>SMLGRLNHVAIAVPDLEKAA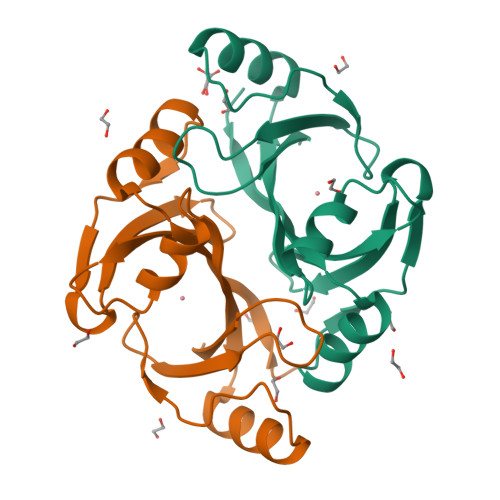AFYKNILGAQVSEAVPLPEHGVSVVFVNLGNTKMELLHPLGLDSPIAGFLQKNKAGGMHHICIEVDNINAAVMDLKKKKIRSLSEEVKIGAHGKPVIFLHPKDCGGVLVELEQA[4x]> SLTSADKSHVKSIWSKASGKAEELGAEAL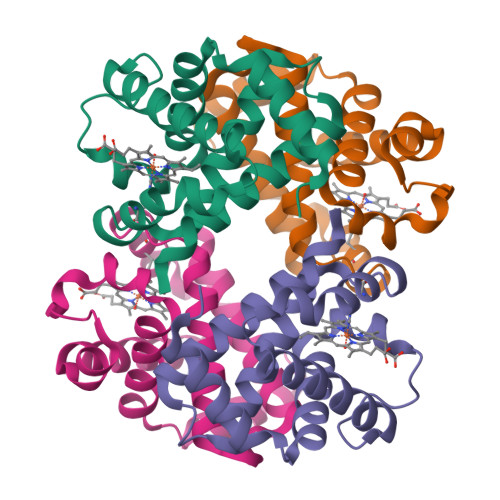GRMLEVFPNTKTYFSHYADLSVSSGQVHTHGKKILDAITTAVNHIDDITGTMTALSTLHAKTLRVDPANFKILSHTILVVLALYFPADFTPEVHLACDKFLASVSHTLATKYR;> EWTDSERFAITTLWAKVNVESVGAQALVRLLVVYPWTQRYFGAFGNISDAAAIAGNAQVHAHGKTVLDSVGNAIAHMDDVADAFTALSTFHSETLHVDPDNFQHFGDCLSIVLAATFGTAYTPDVQAAWQKMIAVIISALSKEYH>[2x]MTYQWLIGIQISLLFVNCICNGSEWSYTNILTGPETWHEHYKNMCSGYYQSPIDLKTDISTLDLKLKTVIIYRNTSSTETTTIQNNGHSAEVKFPRNTWFIS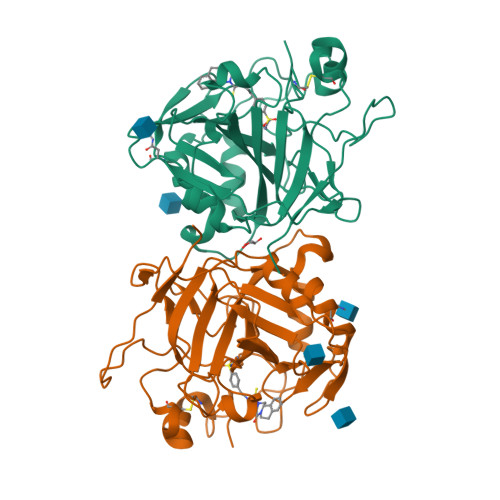FDGILDYKYEIIQMHFHWGNTDDRGSEHTIDGFRFPLEGHIVSFRRQMYSSPSEAIGRPGGLAVLGIMHQIVESIKYEQTAFKAYNNFSGVLNSQFVPPNNSTIDDINLALLLSLLNPSRYFRYLGSLTTPPCTENVLWTVFIDPVLITREQINLFRNLPYGSNEKQTRMGDNFRPIQLLNPIDTLASRTLYRATARSLSLLSLSGILYIMITSQLSVIFL> GATGRTTIAIDPVTRIEGHLKAEVVVENGKVVDARLSGGMYRGFETILRGRDPRDASQIVQRICGVCPTAHSTASVLALDEAFGAKVPNNGRITRNLIFGANYLQSHILHFYHLSAQDFVQGPDTAPFVPRFPKSDLRLSKELNKAGVDQYIEALEVRRICHEMVALFGGRMPHVQGQVVGGATEIPTKEKLVEYAARFKKVRDFVEQKYVPVVYTIGSKYKDMFKVGQGFKAALCVGAFPLDNSGKKHLFMPGVYAKGKDMPFDPSKIKEYVKYSWFAEETTGLNYKEGKTIPAPDKAGAYSFVKAPRYDGLSLEVGPLARMWVNNPELSPVGKKLLKDLFGISAKKFRDLGEEAAFSLMGRHVARAEETYYMLG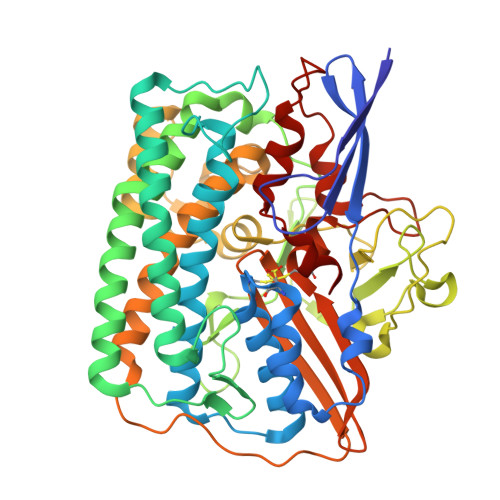AIEGWLKEIKAGEDTVVMPAVPASAEGTGFTEAPRGSLLHYVKVKDSKIDNYQIVSASLWNCNPRDDMGQRGAVEEALIGIPVDDIQNPVNVARLIRAFDPULACAVH> MTTLKLDTLSDRIKAHKNALVHIVKPPVCTERAQHYTEMYQQHLDKPIPVRRALALAHHLANRTIWIKHDELIIGNQASEVRAAPIFPEYTVSWIEKEIDDLADRPGAGFAVSAANARVLHEVCPWWRGQTVQDRCYGMFTDEQKGLLATGIIKAEGNMTSGDAHLAVNFPLLLEKGLDGLREEVAERRSRINLTVLEDLHGEQFLKAIDIVLVAVSEHIERFAALAREMAATETRESRRDELLAMAENCDLIAHQPPQTFWQALQLCYFIQLILQIESNGHSVSFGRMDQYLYPYYRRDVELNQTLDREHAIEMLHSCWLKLLEVNKIRSGSHSKASAGSPLYQNVTIGGQNLVDGQPMDAVNPLSYAILESCGRLRSTQPNLSVRYHAGMSNDFLDACVQVIRCGFGMPAFNNDEIVIPEFIKLGIEPQDAYDYAAIGCIETAVGGKWGYRCTGMSFINFARVMLAALEGGHDATSGKVFLPQEKALSAGNFNNFDEVMDAWDTQIRYYTRKSIEIEYVVDTMLEENVH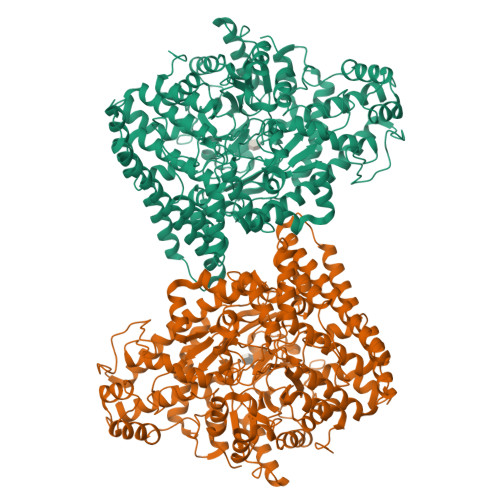DILCSALVDDCIERAKSIKQGGAKYDWVSGLQVGIANLGNSLAAVKKLVFEQGAIGQQQLAAALADDFDGLTHEQLRQRLINGAPKYGNDDDTVDTLLARAYQTYIDELKQYHNPRYGRGPVGGNYYAGTSSISANVPFGAQTMATPDGRKAHTPLAEGASPASGTDHLGPTAVIGSVGKLPTAAILGGVLLNQKLNPATLENESDKQKLMILLRTFFEVHKGWHIQYNIVSRETLLDAKKHPDQYRDLVVRVAGYSAFFTALSPDAQDDIIARTEHML>[2x]GSFTARPSSSMADFRKFFAKAKHIVIISGAGVSAESGVPTFRGAGGYWRKWQAQDLATPLAFAHNPSRVWEFYHYRREVMGSKEPNAGHRAIAECETRLGKQGRRVVVITQNIDELHRKAGTKNLLEIHGSLFKTRCTSCGVVAENYKSPICPALSGKGAPEPGTQDASIPVEKLPRCEEAGCGGLLRPHVVWFGENLDPAILEEVDRELAH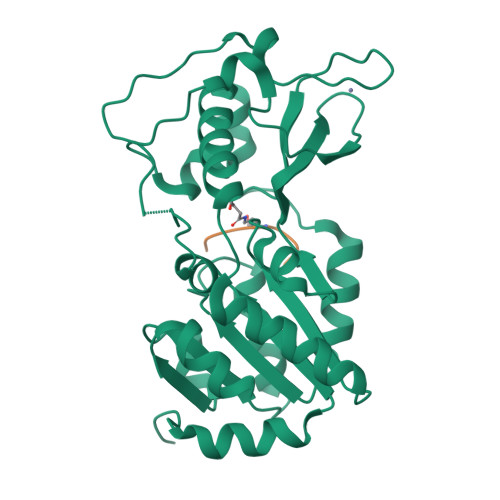CDLCLVVGTSSVVYPAAMFAPQVAARGVPVAEFNTETTPATNRFRFHFQGPCGTTLPEALA;>KQTARXSTGGKA[2x]>[4x]GSRRLLEETLAPFRLNHDQLAAVQAQMRKAMAKGLRGEASSLRMLPTFVRATPDGSERGDFLALDLGGTNFRVLLVRVTTGVQITSEIYSIPETVAQGSGQQLFDHIVDCIVDFQQKQGLSGQSLPLGFTFSFPCRQLGLDQGILLNWTKGFKASDCEGQDVVSLLREAITRRQAVELNVVAIVNDTVGTMMSC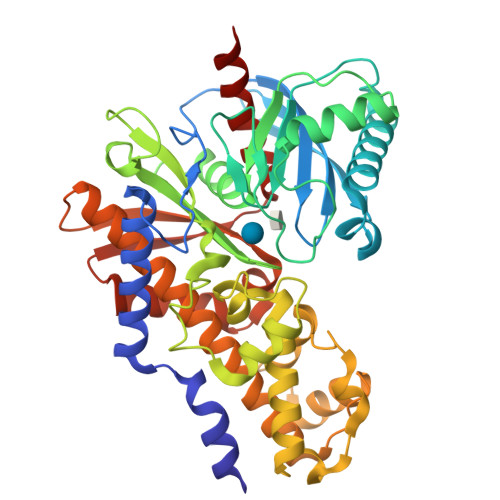GYEDPRCEIGLIVGTGTNACYMEELRNVAGVPGDSGRMCINMEWGAFGDDGSLAMLSTRFDASVDQASINPGKQRFEKMISGMYLGEIVRHILLHLTSLGVLFRGQQIQRLQTRDIFKTKFLSEIESDSLALRQVRAILEDLGLPLTSDDALMVLEVCQAVSQRAAQLCGAGVAAVVEKIRENRGLEELAVSVGVDGTLYKLHPRFSSLVAATVRELAPRCVVTFLQSEDGSGKGAALVTAVACRLAQLTR> MHYRISFIFVTFICLFCFAATGFTQNTNHHHHHHHTDEDSKPVILYSGTPKKYEIADIKVEGVKNYEDYVLIGLSGLSVGQTITVPGDEITGAIKRYWKHGLFSNVQITAEKIEGNKIWLKISLTQRPRIADVRYHGVKKSERTDFESKLGMVKGMQITPNTVDRAKTLIKRYFDDKGFKNAEVIIAQKDDPSNENQVIVDIDIDKKEKIKVHAIHITGNSAIKTSKLKKVMKKTNEKGKLLNLFRTKKFVPENFEADKQLIIDKYNELGYRDAMIVKDSVAQYDEKTVDVYMDIDEGQKYYLRNVTWVGNTLYPSEQLNFLLRMKKGDVYNQKLLGERTS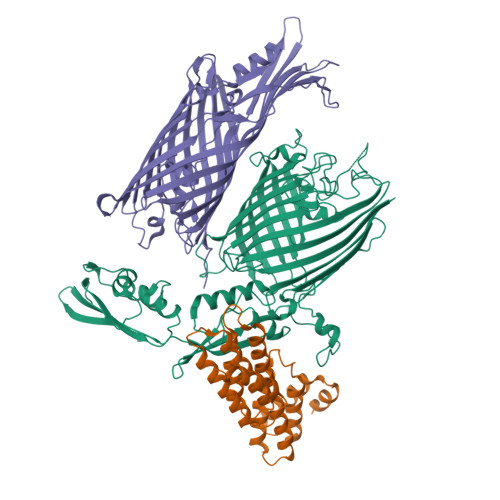TDDDAIGNLYYNNGYLFYNLDPVEVNIVGDSIDLEMRIYEGRQATINKINISGNDRLYENVVRRELRIRPGQLFSKDDLMRSLREIQQMGHFDPEKLQPDIQPDPVNGTVDIGLPLTSKANDQVEFSAGWGQTGIIGKLSLKFTNFSVANLLRPGENYRGILPQGDGQTLTISGQTNAKYYQSYSISFFDPWFGGKRPNSLSVSAFFSVQTDISSRYYNSSYFNNYYNSMYSGYGGYGMYNYGNYNNYENYYDPDKSIKMWGLSLGWGKRLKWPDDYFTLSAELAYQRYNLKDWQYFPVTNGKCNDLSLSLTLARNSIDNPIFPRTGSDFSLSVQLTPPYSLFDGKDYKGYFYDPTDDRGITQDNMNKLHRWVEYHKWKFKAKTYTPLMDYIAHPKCLVLMTRTEFGLLGHYNKYKKSPFGTFDVGGDGMTGYSSYATESIALRGYENSSLTPYGKEGYAYARLGIELRYPLMLETSTNIYVLGFLEAGNAWHDISKFNPFDLKRSAGIGVRIFLPMIGMMGIDWGYGFDKINGSKEYGGSQFHFILGQEF;> MKKNIIITLLAAASLTSCGEYNKLLKSTDYEYKYEAAKNYFAKGQYNRSATLLNELITILKGTDKAEESLYMLGMSYYNQKDYQTAAQTFITYFNTYPRGTFTELARFHAGKSLFLDTPEPRLDQSSTYQAIQQLQMFMEYFPNSTKKQEAQDMIFALQDKLVLKELYSAKLYYNLGNYLGNNYESCVITAQNALKDYPYTDYREELSILILRARHEMAIYSVEDKKMDRYRETIDEYYAFKNEFPESKYLKEAEKIFNESQKVIKD;> MVGFKHTIWALLLMMVTGTAIAQNNTNSPYTRYGYGDLSDQSFGNSKAMGGIAFGLRDGAQINPTNPASYTAIDSLTFLFEGGVSLQNMNISGGGLKLNAKNASFDYLAMQFRLAPWMAMSVGLLPYSNVGYTVSDSQTTDNGLAYSRSFTGDGGLHQMYVGAGVKVLKNLSVGVNASYFWGDITRTRGMFYPGTSSYDSYQRKMVTSISDYKLDFGAQYTQALNKKSSLTIGAVYSPKHKLNNDYTSIVIMGASSSSYGTEYKDVLDATFELPNTFGVGFTYNYDKRLTVGADYSLQQWSKTNFGVVTSDENVRQDFNETFTYCDRTKISVGAEYIPNLIGRSYFAHIKYRLGAYYTTPYYKIDGKKASREYGVTAGFGLPVPRSRSILSISGQFVRVKGLETNMVNENIFRVSIGLTFNERWFFKRRVE>KPIEIIGAPFSKGQPRGGVEKGPAALRKAGLVEKLKETEYNVRDHGDLAFVDVPNDSPFQIVKNPRSVGKANEQLAAVVAETQKNGTISVVLGGDHSMAIGSISGHARVHPDLCVIWVDAHTDINTPLTTSSGNLAGQPVAFLLKELKGKFPDVPGFSWVTPCISAKDIVYIGLRDVDPGEHYIIKTLGIKYFSM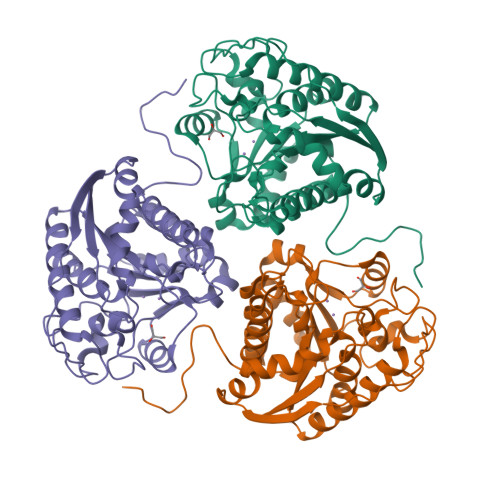TEVDKLGIGKVMEETFSYLLGRKKRPIHLSFDVDGLDPVFTPATGTPVVGGLSYREGLYITEEIYKTGLLSGLDIMEVNPTLGKTPEEVTRTVNTAVALTLSCFGTKREGNHKPETDYL[3x]>MADKIKDAKIIFVVGGPGSGKGTQCEKIVAKYGYTHLSSGDLLRAEVASGSERGKQLQAIMQKGELVPLDTVLDMIKDAMIAKADVSKGFLIDGYPREVKQGEEFEKKIGKPCLLLYVDAKAETMVKRLLKRGETSGRSDDN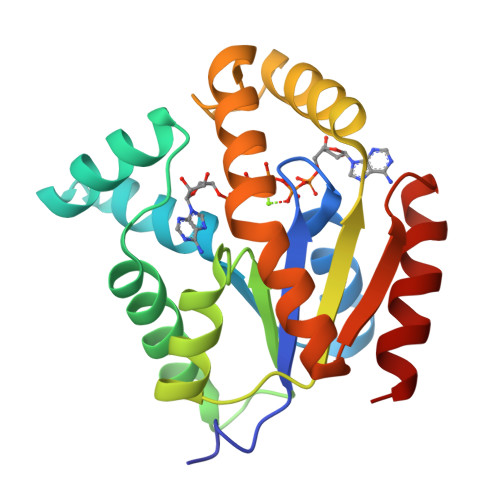EETIKKRLDLYYKATEPVIAFYEGRGIVKKVDSELAVDDVFGQVSKAIDAL[2x]(2S)-N-[(2S)-3-[1-(3-tert-butyl-1-methyl-1H-pyrazole-5-carbonyl)piperidin-4-yl]-1-(methylamino)-1-oxopropan-2-yl]-6-oxopiperidine-2-carboxamide 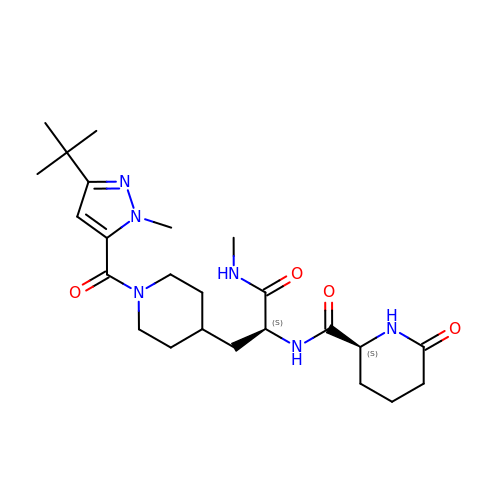| C24 H38 N6 O4 | SLKUTPSFHQUWLD-IRXDYDNUSA-N> MTGGMKPPARKPRILNSDGSSNITRLGLEKRGWLDDHYHDLLTVSWPVFITLITGLYLVTNALFALAYLACGDVIENARPGSFTDAFFFSVQTMATIGYGKLIPIGPLANTLVTLEALCGMLGLAVAASLIYARFTRPTAGVLFSSRMVISDFEGKPTLMMRLANLRIEQIIEADVHLVLVRSEISQEGMVFRRFHDLTRTRSRSPIFSLSWTVMHPIDHHSPIYGETDETLRNSHSEFLVLFTGHHEAFAQNVHARHAYSCDEIIWGGHFVDVFTT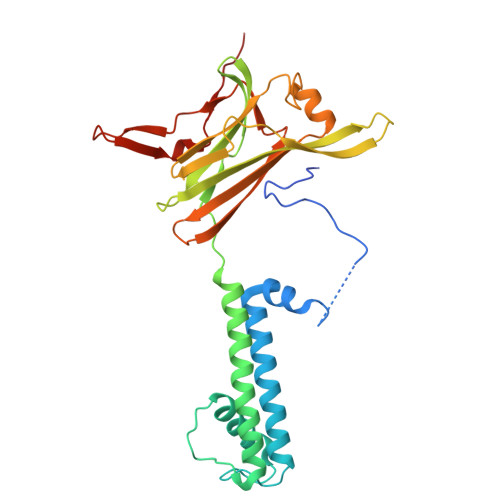LPDGRRALDLGKFHEIAQHHHHHH Enzyme rhodopsins comprise the N-terminal rhodopsin domain and C-terminal enzyme domain, connected by a linker, and function as light-activated enzymes. Rh-PDE derived from Salpingoeca rosetta (SrRh-PDE) was first identified and exhibits light-dependent hydrolytic activity for both of cAMP and cGMP, whereas it lacks pump or channel activity. SrRh-PDE consists of the long N-terminal region, transmembrane domain (TMD), including the rhodopsin domain, C-terminal PDE domain, and 76-residue linker region connecting the TMD and PDE domain. Here, we present crystal structures of SrRh-PDE–TMD with and without the linker region, at 3.5 and 2.6 Å resolutions, respectively.

We next determined the 2.1 Å resolution crystal structure of the PDE domain with the linker region (Linker–PDE, residues 347–703). The N-terminal residues Lys380–Met386 are newly observed as compared with the reported structure, while residues 347–379 are disordered. The Ala385 backbone amide forms a hydrogen bond with the Glu478 sidechain, fixing the N-terminal residues and extending toward the dimer interface. The TMD–Linker and Linker–PDE structures provided insights into their connectivity, but there is no observed density to assign residues 354–379 in the linker region. The C-terminal residues 380–386 in the third α-helix were unwound, as similarly in our Linker–PDE structure.

> MDDDVKSWIMNEFSGSTDGKGGDDAKAQQRARGRKGHSAAMDAEKLAASSLFTWDFDALDKSDEDLTAVCVRVFQELHVIEQFNIDEKKLRKWLQKVRTQYNKNPFHNWRHAVMVLHTTYLLLTSVATEFITEVELLAMLIAALSHDLDHNGLTNAFHINSRSELALVYNDQSVLENHHSHLAFEILLEKGCNVVENLDEDEFKRLRAVIINCILNTDMATHHTKLSKMEEVNRLGGFINLAENNDQRLFVLAVLLHTADLHNPIKPFESNKRWSARLQKEFNNQVELEAKMNLPSLPFMRGNDEESLAKGEIGFINFVVKPWHQQLSQAFPKLDFLLDTIDANLAEWKAIAESYRQMQENLYFQ> MRSIYLCRHGESELNLRGRIGGDSGLSARGKQYAYALANFIRSQGISSLKVWTSHMKRTIQTAEALGVPYEQWKALNEIDAGVCEEMTYEEIQEHYPEEFALRDQDKYRYRYPKGESYEDLVQRLEPVIMELERQENVLVICHQAVMRCLLAYFLDKSSDELPYLKCPLHTVLKLTPVAYGCRVESIY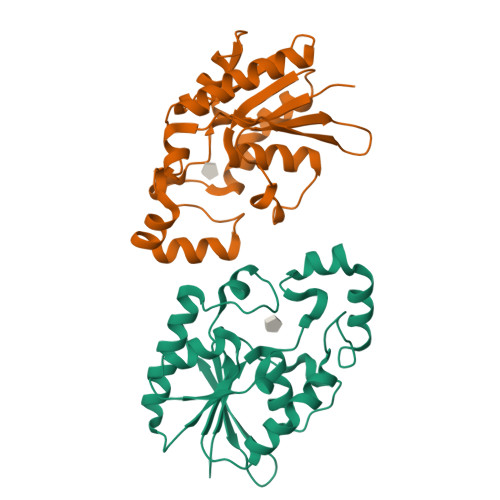LNV(HYDROXYETHYLOXY)TRI(ETHYLOXY)OCTANE | C16 H34 O5 | 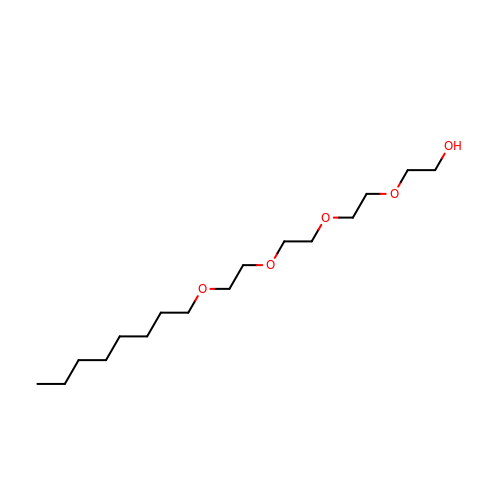FEOZZFHAVXYAMB-UHFFFAOYSA-N5-azanyl-4-oxidanylidene-pentanoic acid | C5 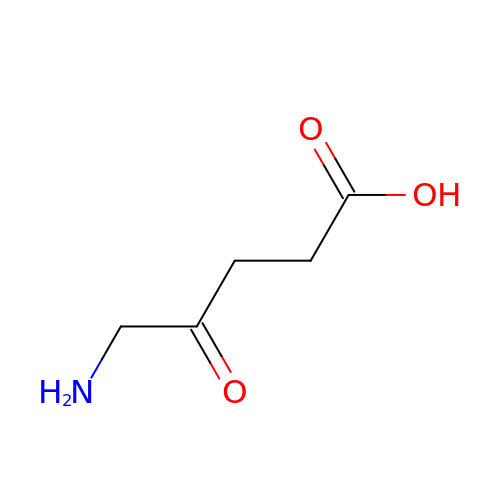H9 N O3 | ZGXJTSGNIOSYLO-UHFFFAOYSA-N6-O-phosphono-beta-D-galactopyranose 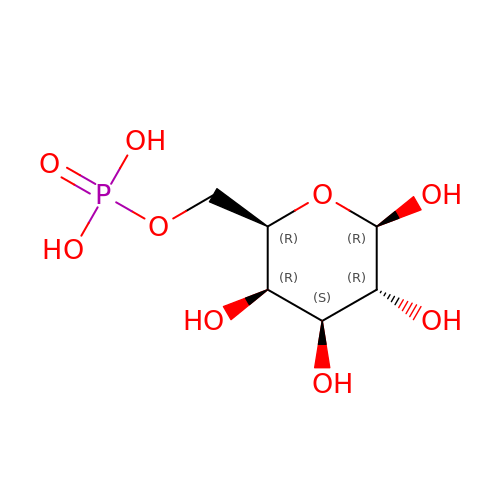| C6 H13 O9 P | NBSCHQHZLSJFNQ-FPRJBGLDSA-N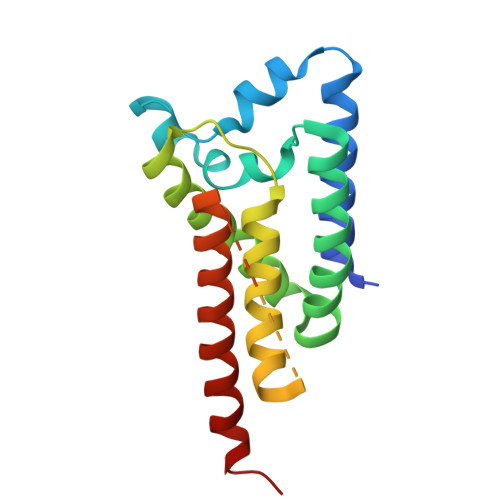> MENFLAQQGKITLILTALCVLIYIAQQLGFEDDIMYLMHYPAYEEQDSEVWRYISHTLVHLSNLHILFNLSWFFIFGGMIERTFGSVKLLMLYVVASAITGYVQNYVSGPAFFGLSGVVYAVLGYVFIRDKLNHHLFDLPEGFFTMLLVGIALGFISPLFGVEMGNAAHISGLIVGLIWGFIDSKLRKNSLELVPR> ESKSFAVGMFKGQLTTDQVFPYPSVLNEEQTQFLKELVEPVSRFFEEVNDPAKNDALEMVEETTWQGLKELGAFGLQVPSELGGVGLCNTQYARLVEIVGMHDLGVGITLGAHQSIGFKGILLFGTKAQKEKYLPKLASGETVAAFCLTEPSSGSDAASIRTSAVPSPCGKYYTLNGSKLWISNGGLADIFTVFAKTPVTDPATGAVKEKITAFVVERGFGGITHGPPEKKMGIKASNTAEVFFDGVRVPSENVLGEVGSGFKVAMHILNNGRFGMAAALAGTMRGIIAKAVDHATNRTQFGEKIHNFGLIQEKLARMVMLQYVTESMAYMVSANMDQGATDFQIEAAISKIFGSEAAWKVTDECIQIMGGMGFMKEPGVERVLRDLRIFRIFEGTNDILRLFVALQGCMDKGKELSGLGSALKNPFGNAGLLLGEAGKQLRRRAGLGSGLSLSGLVHPELSRSGELAVRALEQFATVVEAKLIKHKKGIVNEQFLLQRLADGAIDLYAMVVVLSRASRSLSEGHPTAQHEKMLCDT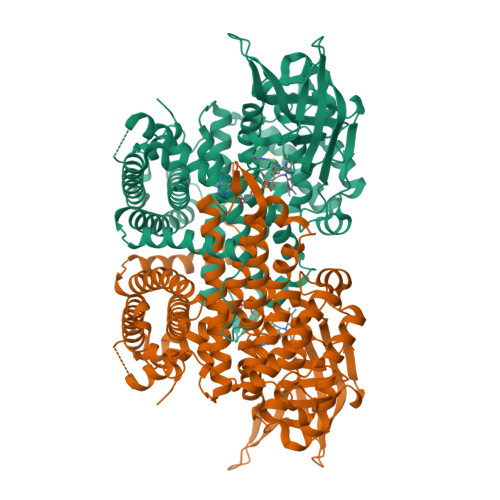WCIEAAARIREGMAALQSDPWQQELYRNFKSISKALVERGGVVTSNPLGF> MFVRVMKIAQNKKIVTVYPTTTIRKALMTMNENKYRRLPVVNAGNNKVVGIITSMDIVDFMGGGSKYNLIREKHERNFLAAINEPVREIME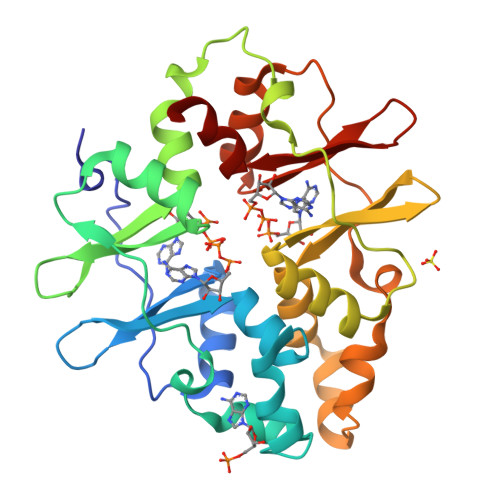ENVITLKENADIDEAIETFLTKNVGGAPIVNDENQLISLITERDVIRALLDKIDENEVIDDYITRDVIVATPGERLKDVARTMVRNGFRRLPVVSEGRLVGIITSTDFIKLLGSDWAFNHMQTGNVREITNVRMEEIMKRDVITAKEGDKLKKIAEIMVTNDIGALPVVDENLRIKGIITEKDVLKYFA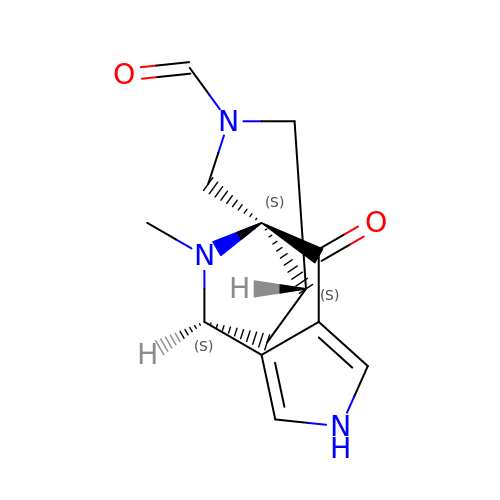(3aS,8S,9aS)-10-methyl-4-oxo-1,4,6,8,9,9a-hexahydro-3a,8-epiminocyclohepta[1,2-c:4,5-c']dipyrrole-2(3H)-carbaldehyde | C13 H15 N3 O2 | HQZKECRFEYSMAO-LJUAHTATSA-N> MGHHHHHHGSLVPRGSDVQELNSIIQRISKFDNILKDKTIINQQDLRQISWNGIPKIHRPVVWKLLIGYLPVNTKRQEGFLQRKRKEYRDSLKHTFSDQHSRDIPTWHQIEIDIPRTNPHIPLYQFKSVQNSLQRILYLWAIRHPASGYVQGINDLVTPFFETFLTEYLPPSQIDDVKIKDPSTYMVDEQITDLEADTFWCLTKLLEQITDNYIHGQPGILRQVKNLSQLVKRIDADLYNHFQN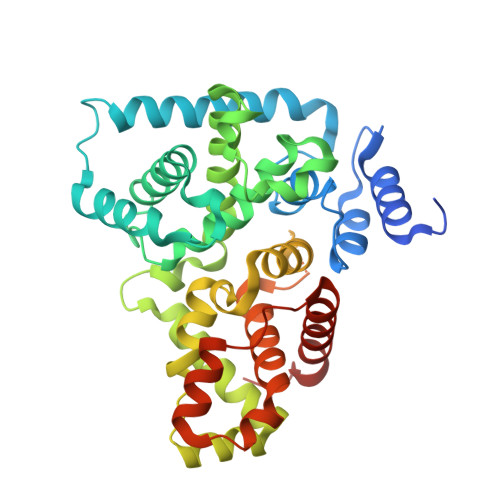EHVEFIQFAFRWMNCLLMREFQMGTVIRMWDTYLSETSQEVTSSYSMSSNDIKPPVTPTEPRVASFVTPTKDFQSPTTALSNMTPNNAVEDSGKMRQSSLNEFHVFVCAAFLIKWSDQLMEMDFQETITFLQNPPTKDWTETDIEMLLSEAFIWQSLYKDATSHWL imidazo[1,2-a]pyridin-5-amine 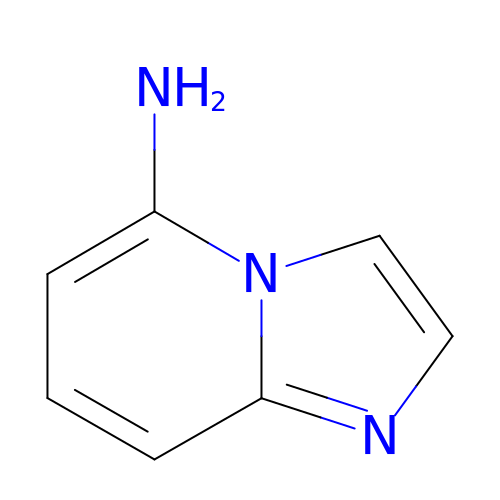| C7 H7 N3 | XSNBOUDHWWROII-UHFFFAOYSA-N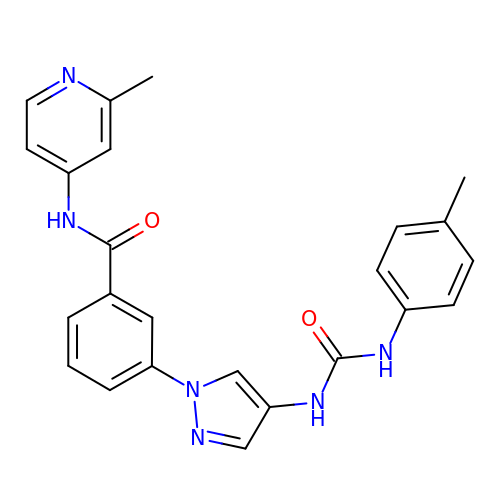3-(4-{[(4-methylphenyl)carbamoyl]amino}-1H-pyrazol-1-yl)-N-(2-methylpyridin-4-yl)benzamide | C24 H22 N6 O2 | BMQOTQLVHNKQRK-UHFFFAOYSA-N> MENIDLPQGLVNFSTQHLQLIRFKAGLNETVLPGVEAIGLGYNPFISYASVNSGAVQLFDWATAKKREVPFKAGYFVPELVDVQQNDSATFTNVSGNTLSEYQRSLATSVAIEGRYNFFSGSLSTDFDSNSLRNAENEFTRIQQSINLWSLRLPSVKSLRELMLPHMRQQLDELNVNDPKAISRYFDRVGSHFLTGIVMGGRAILASSTNKLRVKRDYSVSVVAKASYEGLTGQLSAEAKAKYGESISSFTQYSNTHQEVRGGDGAKAHGVFSGKKEDFQAWVDSVSASPDFVDFVPTIPMQEIWTLCSSEAQAEAMRKHFDDVWAPAQSEKFRVKANFIDQLVVLTGGSSTIEPPVGYSKIEYDLNAGAGGDFIYLCYHEQTWQADRPKDAVTDIRIIFNKEPTPPGYTKLPQDLNKGAGGDDVFLCYKTEAFNTDTAINKVTVIGGNNADLNAPYGYLKVPGDLNRGAGGNFIYACTFVGK

Mpf2Ba1 is a 53.2 kDa protein isolated from Pseudomonas monteilii through a multi-step purification process informed by artificial diet bioactivity screening against WCR larvae. The protein is comprised of two domains—an N-terminal MACPF domain and a C-terminal β-prism domain. Pore-forming proteins (PFPs) are a major class of soluble proteins that oligomerize into rings and undergo large irreversible conformational changes to become transmembrane assemblies and breach the membrane of target cells. We have identified and characterized the non-Bt insecticidal protein Mpf2Ba1, providing mechanistic details for how it effectively kills the devastating maize pest WCR by forming pores in midgut membranes targeting a different binding site than the insecticidal proteins currently deployed in commercial transgenic maize hybrids.

We first solved the X-ray structure of Mpf2Ba1-1167 at 2.1 Å resolution. The MACPF domain has a central four-stranded antiparallel β-sheet with a characteristic ~90° bend. The β-sheet is interrupted by three insertions: two sets of transmembrane hairpins emerge from its base (TMH1, buried inside the hydrophobic core, and TMH2, facing the surface), and a helix-turn-helix (HTH) motif, harboring several residues that are highly conserved in all known MACPF/CDCs15, intercalates at the bend of strand β4. In Mpf2Ba1, each of the three β-sheets of the β-prism, arranged around a local three-fold axis, contains a unique repeated motif: Asp-Leu-Asn (DLN). These DLN motifs create an octahedral geometry coordinating a Mg2+ at the symmetry axis through the Leu carbonyl oxygen and the Asn side-chain amide oxygen. Structurally, the metal chelation seems to tuck the three β-prism loops into gaps between the adjacent β-sheets, increasing domain stability. In the monomer, the N-terminus lies adjacent to one side of the MACPF domain, forming a short β-strand–β-sheet interaction with the central β-sheet, and two more H-bonds: between Asp292, stabilized by the conserved Pro291, and the N-terminal backbone, and between one of the nitrogen atoms of N-terminal His18 imidazole ring and the oxygen atom of Ser54, highly conserved among bacterial MACPFs. Since we observed that some of these residues are involved in intermolecular contacts with the neighboring subunit, we think that the steric hindrance imposed by the N-terminus could prevent premature interactions/oligomerization of soluble monomers. The X-ray density for this loop is clear, albeit weaker and with higher B-factors than the surrounding residues, indicating greater flexibility. We solved the Mpf2Ba1 X-ray structure and showed how N-terminal residues inhibit the association of monomers in the soluble form.Here, we characterize the O-methyltransferases BelI and CysG, which catalyze the initial step of β-lactone formation. Employing techniques such as crystallography, computational analysis, mutagenesis, and activity assays, we identified a His-His-Asp (HHD) motif in the active sites of the two enzymes, which is crucial for binding a catalytically active calcium ion. As expected, BelI as well as CysGΔN16 adopt the class I methyltransferase Rossmann fold, characterized by a core domain of a seven-stranded β-sheet flanked by α-helices. The HHD-motif enables regiospecific C1-carboxy group methylation of their respective malic substrates.

Conservative asparagine replacements in the HHD motif resulted in CysG variants that remained active. CysGfl-D191N showed a 56% decrease in substrate turnover, while CysGfl-H122N and CysGfl-H123N were fully active compared to wt but were inactivated with EDTA. Strikingly, the CysGfl-H123N variant showed 91% of the original catalytic activity with Ca2+, whereas Mg2+ and Mn2+ resulted in only 50% residual activity. Analysis of the complex geometry in high-resolution structures, X-ray fluorescence measurements, as well as metal-dependent activity assays with the CysGfl-H123N variant indicate Ca2+ as the intrinsically bound metal ion.

>[2x]GSTYDALRRQLIPSFDLLYGSAVSVVAMSVPATARILDLGAGTGLLGAALRERLPDAELLLQDRSQAMLEQARQRFADDDQVAIRVADHLDELPAGPFDAVVSALSIHNLEHQDKQDLFTRIRKILRPGGIFVNVEQVLAPTSELEKMYDRQHEAHVLASDTPAEEWAAGRERMKHDIPIDVETQIQWLRDAGFTTADCLAKDWRFATYAGWNGS>MQFTKCELSQLLKDIDGYGGIALPELICTMFHTSGYDTQAIVENNESTEYGLFQISNKLWCKSSQVPQSRNICDISCDKFLDDDITDDIMCAKKIL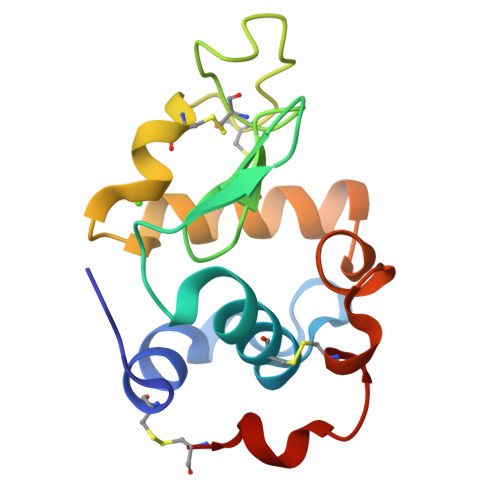DIKGIDYWLAHKALCTEKLEQWLCEKL[2x]>MNDSSVIYRAIVTSKFRTEKMLNFYNSIGSGPDKNTIFITFGRSEPWSSNENEVGFAPPYPTDSVLGVTDMWTHMMGTVKVLPSMLDAVIPRRDWGDTRYPDPYTFRINDIVVCNSAPYNATESGAGWLVYRCLDVPDTGMCSIASLTDKDECLKLGGKWTPSARSMTPPEGRGDAEGTIEPGDGYVWEYLFEIPPDVSINRCTNEYIVVPWPEELKEDPTRWGYEDNLTWQQDDFGLIYRVKANTIRFKAYLDSVYFPEAALPGNKGFRQISIITNPLEAKAHPNDPNVKAEKDYYDPEDLMRHSGEMIYMENRPPIIMAMDQTEEINILFTF[2x];>MFIQEPKKLIDTGEIGNASTGDILFDGGNKINSDFNAIYNAFGDQRKMAVANGTGADGQIIHATGYYQKHSITEYATPVKVGTRHDIDTSTVGVKVIIERGELGDCVEFINSNGSISVTNPLTIQAIDSIKGVSGNLVVTSPYSKVTLRCISSDNSTSVWNYSIESMFGQKESPAEGTWNISTSGSVDIPLFHRTEYNMAKLLVTCQSVDGRKIKTAEINILVDTVNSEVISSEYAVMRVGNET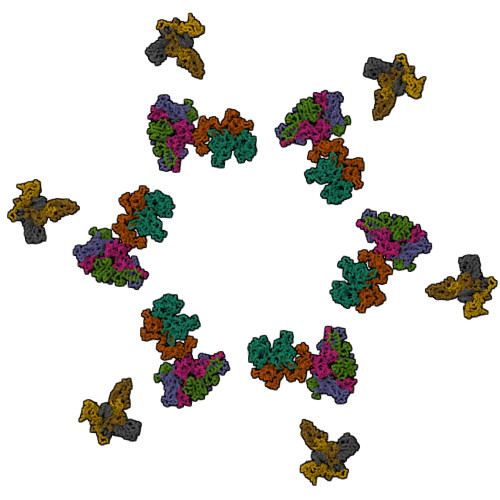EEDEIANIAFSIKENYVTATISSSTVGMRAAVKVIATQKIGVAQ[3x];>MSLLNNKAGVISRLADFLGFRPKTGDIDVMNRQSVGSVTISQLAKGFYEPNIESAINDVHNFSIKDVGTIITNKTGVSPEGVSQTDYWAFSGTVTDDSLPPGSPITVLVFGLPVSATTGMTAIEFVAKVRVALQEAIASFTAINSYKDHPTDGSKLEVTYLDNQKHVLSTYSTYGITISQEIISESKPGYGTWNLLGAQTVTLDNQQTPTVFYHFERTA[3x]> MGHHHHHHMSADFGLIGLAVMGQNLIL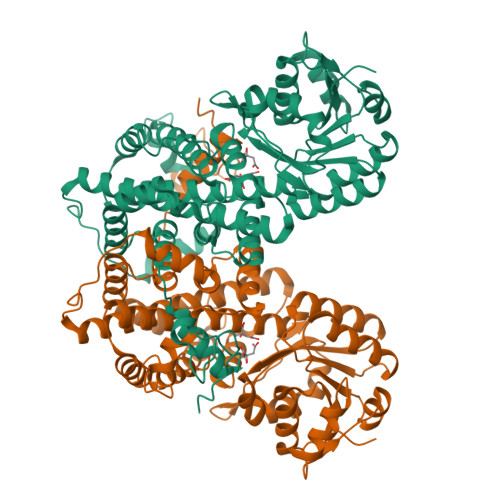NAADHGFTVCAYNRTQSKVDHFLANEAKGKSIIGATSIEDFISKLKRPRKVMLLVKAGAPVDALINQIVPLLEKGDIIIDGGNSHFPDSNRRYEELKKKGILFVGSGVSGGEEGARYGPSLMPGGSEEAWPHIKNIFQSISAKSDGEPCCEWVGPAGAGHYVKMVHNGIEYGDMQLICEAYDIMKRLGGFTDKEISDVFAKWNNGVLDSFLVEITRDILKFDDVDGKPLVEKIMDTAGQKGTGKWTAINALDLGMPVTLIGEAVFARCLSALKNERIRASKVLPGPEVPKDAVKDREQFVDDLEQALYASKIISYAQGFMLIREAAATYGWKLNNPAIALMWRGGCIIRSVFLGQITKAYREEPDLENLLFNKFFADAVTKAQSGWRKSIALATTYGIPTPAFSTALSFYDGYRSERLPANLLQAQRDYFGAHTFRVLPECASDNLPVDKDIHINWTGHGGNVSSSTYQA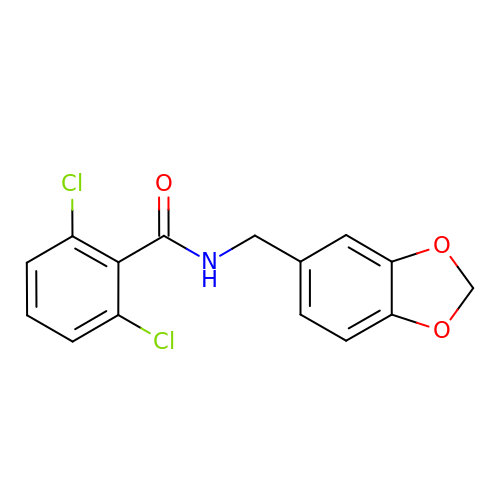N-(1,3-benzodioxol-5-ylmethyl)-2,6-dichlorobenzamide | C15 H11 Cl2 N O3 | NMKJFZCBCIUYHI-UHFFFAOYSA-N> MSLRSEQEMMDIFLDFALNDERIRLVTLEGSRTNRNIPPDNFQDYDISYFVTDVESFKENDQWLEIFGKRIMMQKPEDMELFPPELGNWFSYIILFEDGNKLDLTLIPIREAEDYFANNDGLVKVLLDKDSFINYKVTPNDRQYWIKRPTAREFDDCCNEFWMVSTYVVKGLARNEILFAIDHLNEIVRPNLLRMMAWHIASQKGYSFSMGKNYKFMKRYLSNKEWEELMSTYSVNGY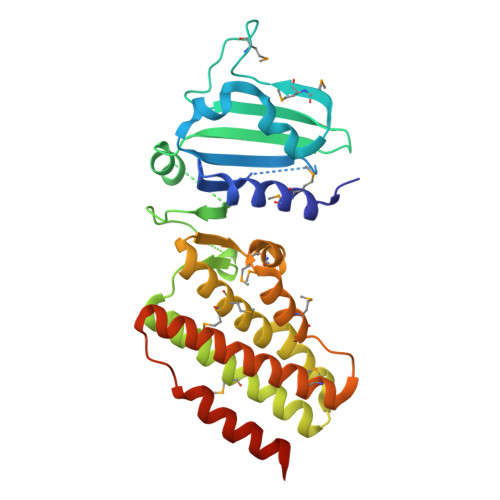QEMWKSLFTCYALFRKYSKAVSEGLAYKYPDYDEGITKYTEGIYCSVKEGHHHHHH>MVYMAINAVAGTIREFSPKDIESVYRIAQTSLTEYYTQALILDLHREWPESFMVYTVAGSVVGFIVGSKYSRTEARILLFAVDERFRRMGVGSALMDAFLSLCREQNMLSVRLEVRTDNDEAIRFYKKYGFVI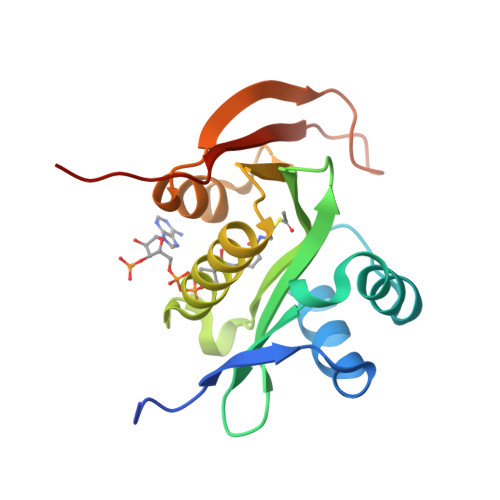TAMLPNYYSDSSNAYTMWRIVLEHHHHHH[16x]>[3x]GPHMFEARLVQGSILKKVLEALKDLINEACWDISSSGVNLQSMDSSHVSLVQLTLRSEGFDTYRCDRNLAMGVNLTSMSKILKCAGNEDIITLRAEDNADTLALVFEAPNQEKVSDYEMKLMDLDVEQLGIPEQEYSCVVKMPSGEFARICRDLSHIGD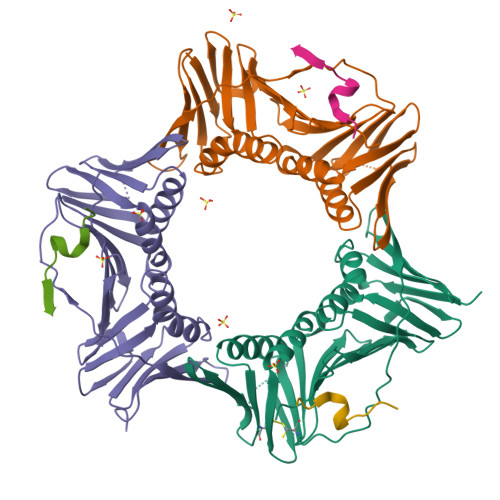AVVISCAKDGVKFSASGELGNGNIKLSQTSNVDKEEEAVTIEMNEPVQLTFALRYLNFFTKATPLSSTVTLSMSADVPLVVEYKIADMGHLKYYLAPKIEDEEGS;>[3x]MGRKRLITDSYPVVKRREG> GRKEPEIITVTLKKQNGMGLSIVAAKGAGQDKLGIYVKSVVKGGAADVDGR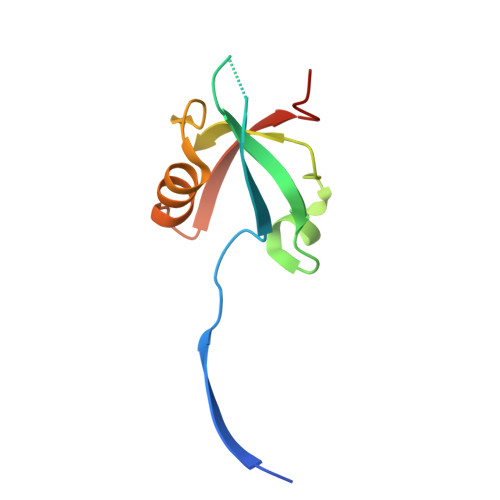LAAGDQLLSVDGRSLVGLSQERAAELMTRTSSVVTLEVAKQGAIYH> MTQPLVGKQILIVEDEQVFRSLLDSWFSSLGATTVLAADGVDALELLGGFTPDLMICPIAMPRMNGLKLLEHIRNRGDQTPVLVISATENMADIAKALRLGVEDVLLKPVKDLNRLREMVFACLYPSMFNSRVEEEERLFRDWDAMVDNPAAAA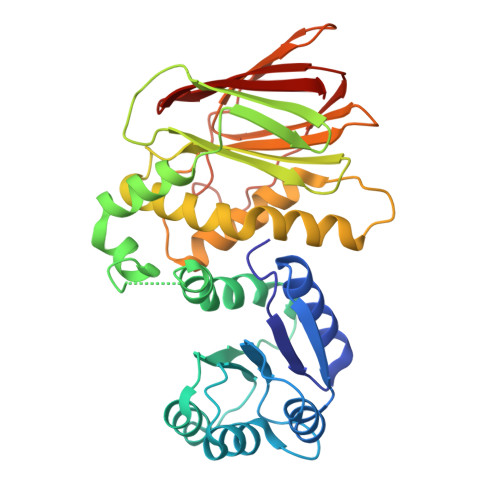KLLQELQPPVQQVISHCRVNYRQLVAADKPGLVLDIAALSENDLAFYCLDVTRAGHNGVLAALLLRALFNGLLQEQLAHQNQRLPELGALLKQVNHLLRQANLPGQFPLLVGYYHRELKNLILVSAGLNATLNTGEHQVQISNGVPLGTLGNAYLNQLSQRCDAWQCQIWGTGGRLRLMLSAE>SNAMLIIETLPLLRQHIRRLRQEGKRVALVPTMGNLHDGHMKLVDEAKARAD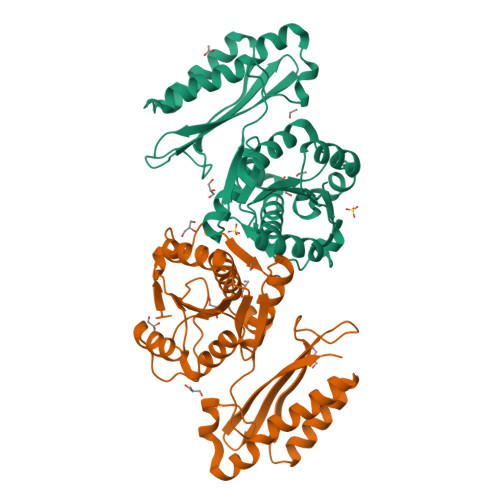VVIVSIFVNPMQFDRPDDLVRYPRTLQEDCEKLNKRKVDYVFAPAVEEIYPHGLEGQTYVDVPGLSTMLEGASRPGHFRGVSTIVSKLFNLIQPDIACFGEKDFQQLALIRKMVADMSYDIEIVGVPIIRAKDGLALSSRNAYLTAEQRKIAPGLYNVMNSIAEKLIAGNRELQEIIAIAEQELNEKGFRADDIQIRDADTLLELTETSKRAVILAAAWLGQARLIDNQSVTLAQ[4x]5-(4,4-DIMETHYL-2-THIOXO-1,4-DIHYDRO-2H-3,1-BENZOXAZIN-6-YL)-1-METHYL-1H-PYRROLE-2-CARBONITRILE | C16 H15 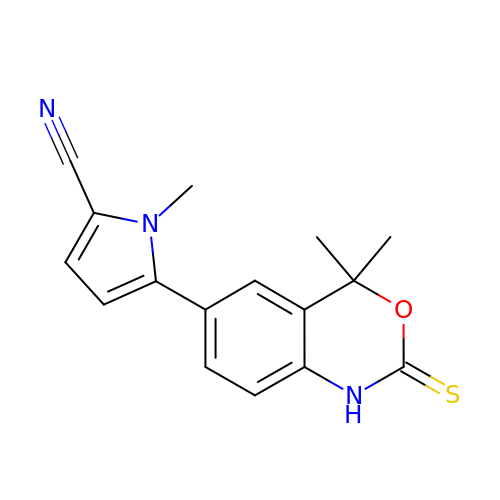N3 O S | PYVFWTPEBMRKSR-UHFFFAOYSA-N Striga seeds require host-derived strigolactones (SLs) for germination, and corresponding antagonists could be used as germination inhibitors. In Striga, the receptors responsible for SL-induced seed germination are evolutionarily derived from a KARRIKIN INSENSITIVE 2 (KAI2) receptor and have arisen through gene duplication and new functionalization replacing the karrikin ligand by SLs. Among the several Striga SL receptors, S. hermonthica HYPO-SENSITIVE TO LIGHT (ShHTLs), ShHTL7 is the most sensitive to SLs. It is assumed to play a crucial role in regulating Striga seed germination.

Previously, the structure of ShHTL7, co-crystallized with Triton X-100, showed that the hydrophobic tail of the ligand, which includes the phenoxy group, interacts with several amino acids in the receptor cavity. These interactions provide the basis for the tight binding of Triton X-100 and its blocking/inhibition activity, together with those that take place with the polyethylene repeats at the outer rim of the ShHTL7 binding pocket. Building upon this work, we co-crystallized ShHTL7 with the triazole urea derivative KK007, after incubating them together, and soaked the obtained crystal in 1 mM Triton X-100 solution. Thus, we determined a crystal structure that showed KK007and Triton X-100 bound to ShHTL7, where KK007 was covalently linked to the catalytic Ser95. This structure showed that Triton X-100 left enough space in the active site to accommodate small covalent ligands targeting Ser95, and, hence, suggested that the combination of both moieties might generate efficient and Striga-specific inhibitors. Therefore, we attached the alkyl benzene moiety, which corresponds to the hydrophobic tail of Triton X-100 without the methyl groups, to the triazole urea scaffold, which led to the two compounds KK023-N1 and KK023-N2. The presence of the triazole urea scaffold in KK023-N1 and -N2 makes covalent binding to the active site serine in ShHTL7 likely, as shown for KK007 and the D14 inhibitor KK094. Our docking model of KK023-N1 bound to ShHTL7 also suggests that the compound does not reach deep enough in the ShHTL7 binding pocket to use its potential for covalent linkage with the catalytic Ser95. Structure analysis revealed that ShHTL7 possesses a large ligand-binding pocket among other SL receptors in parasitic and nonparasitic plants. Also, the ShHTL7 binding pocket is composed of nonbulky residues, compared to OsD14 and ShHTL5, and this explained the basis for the ligand selectivity.

> GPLGSMSSIGLAHNVTILGSGETTVVLGHGYGTDQSVWKLLVPYLVDDYKVLLYDHMGAGTTNPDYFDFDRYSSLEGYSYDLIAILEEFQVSKCIYVGHSMSSMAAAVASIFRPDLFHKLVMISPTPRLINTEEYYGGFEQKVMDETLRSLDENFKSLSLGTAPLLLACDLESAAMQEYCRTLFNMRPDIACCITRMICGLDLRPYLGHVTVPCHIIQSSNDIMVPVAVGEYLRKNLGGPSVVEVMPTEGHLPHLSMPEVTIPVVLRHIRQDITDH> GAMGLPEEPSSPQESTLKALSLYEAHLSSYIMYLQTFLVKTKQKVNNKNYPEFTLFDTSKLKKDQTLKSIKTNIAALKNHIDK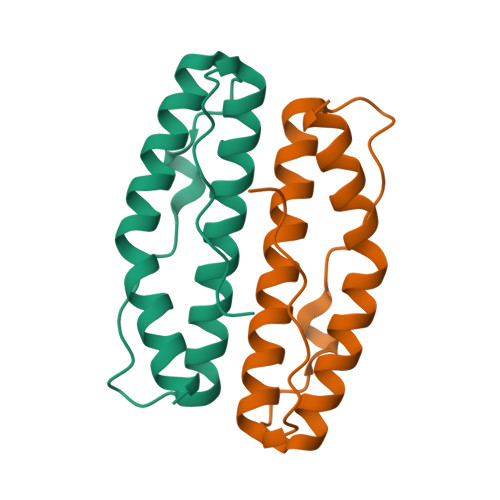IKPIAMQIYKKYSKNIP>[2x]MSANDK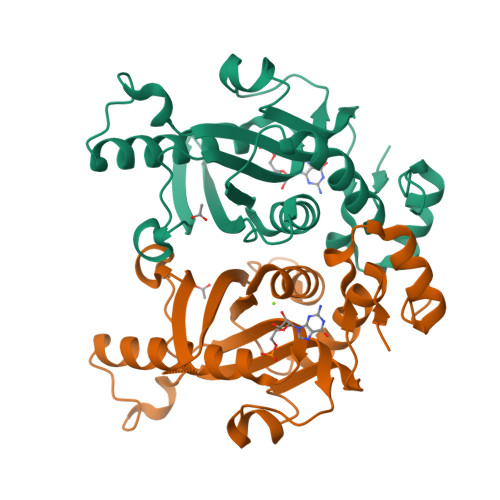QYISYNNVHQLCQVSAERIKNFKPDLIIAIGGGGFIPARILRTFLKEPGVPTIRIFAIILSLYEDLNSVGSEVEEVGVKVSRTQWIDYEQCKLDLVGKNVLIVDEVDDTRTTLHYALSELEKDAAEQAKAKGIDTEKSPEMKTNFGIFVLHDKQKPKKADLPAEMLNDKNRYFAAKTVPDKWYAYPWESTDIVFHTRMAIEQGNDIFIPEQEHKQ>MSHVELQPGFDFQQAGKEVLAIERECLAELDQYINQNFTLACEKMFWCKGKVVVMGMGASGHIGRKMAATFASTGTPSFFVHPGEAAHGDLGMVTPQDVVIAISNSGESSEITALIPVLKRLHVPLICITGRPESSMARAADVHLCVKVA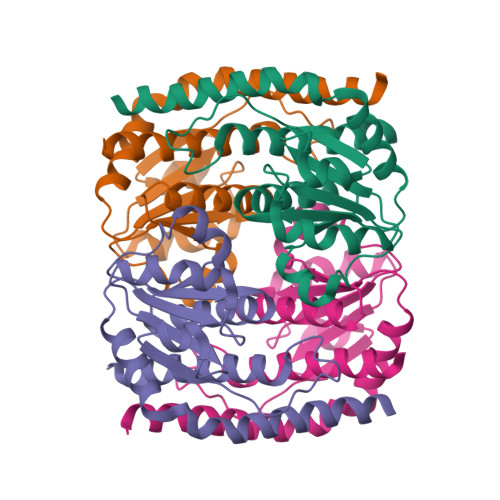KEACPLGLAPTSSTTATLVMGDALAVALLKARG[4x]> EPLDDYVNTQGASLFSVTKKQLGAGSIEECAAKCEEDEEFTCRAFQYHSKEQQCVIMAENRKSSIIIRMRDVVLFEKKVYLSECKTGNGKNYRGTMSKTKNGITCQKWSSTSPHRPRFSPATHPSEGLEENYCRNPDNDPQGPWCYTTDPEKRYDYCDILECEEECMHCSGENYDGKISKTMSGLECQAWDSQSPHAHGYIPSKFPNKNLKKNYCRNPDRELRPWCFTTDPNKRWELCDIPRCTTPPPSSGPTYQCLKGTGENYRGNVAVTVSGHTCQHWSAQTPHTHNRTPENFPCKNLDENYCRNPDGKRAPWCHTTNSQVRWEYCKIPSCDSSPVSTEQLAPTAPPELTPVVQDCYHGDGQSYRGTSSTTTTGKKC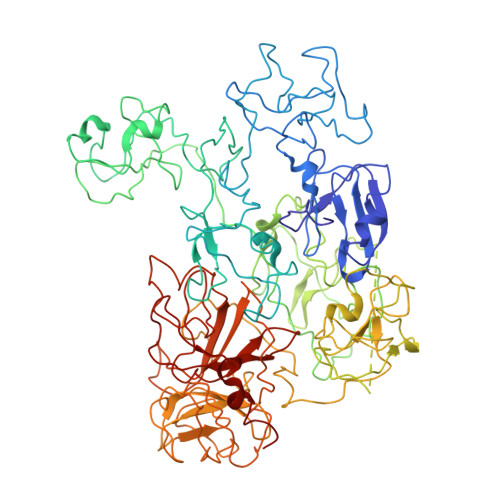QSWSSMTPHRHQKTPENYPNAGLTMNYCRNPDADKGPWCFTTDPSVRWEYCNLKKCSGTEASVVAPPPVVLLPDVETPSEEDCMFGNGKGYRGKRATTVTGTPCQDWAAQEPHRHSIFTPETNPRAGLEKNYCRNPDGDVGGPWCYTTNPRKLYDYCDVPQCAAPSFDCGKPQVEPKKCPGRVVGGCVAHPHSWPWQVSLRTRFGMHFCGGTLISPEWVLTAAHCLEKSPRPSSYKVILGAHQEVNLEPHVQEIEVSRLFLEPTRKDIALLKLSSPAVITDKVIPACLPSPNYVVADRTECFITGWGETQGTFGAGLLKEAQLPVIENKVCNRYEFLNGRVQSTELCAGHLAGGTDSCQGDSGGPLVCFEKDKYILQGVTSWGLGCARPNKPGVYVRVSRFVTWIEGVMRNN> MIAQQHKDTVAACEAAEAIAIAKDQVWDGEGYTKYTFDDNSVLIQSGTTQYA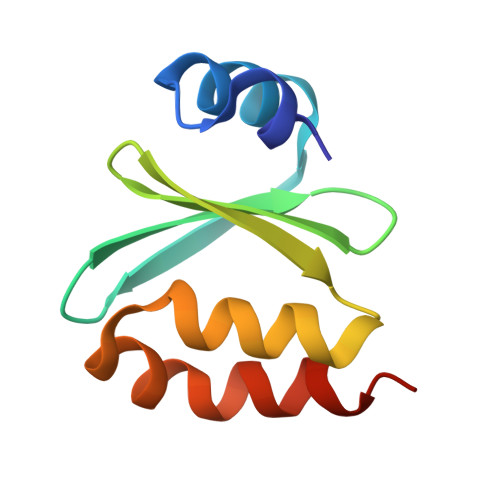MDADDADSIKGYADWLDDEARSAEASEIERLLESVEEE>CPRFLKVKNWETDVVLTDTLHLKSTLETGCTEHICMGSIMLPSQHTRKPEDVRTKDQLFPLAKEFLDQYYSSIKRFGSKAHMDRLEEVNKEIESTSTYQLKDTELIYGAKHAWRNASRCVGRIQWSKLQVFDARDCTTAHGMFNYICNHVKYATNKGNLRSAITIFPQRTDGKHDFRVWNSQLIRYAGYKQPDGSTLGDPANVQFTEICIQQGWKAPRGRFDVLPLLLQANGNDPELFQIPPELVLEVPIRHPKFDWFK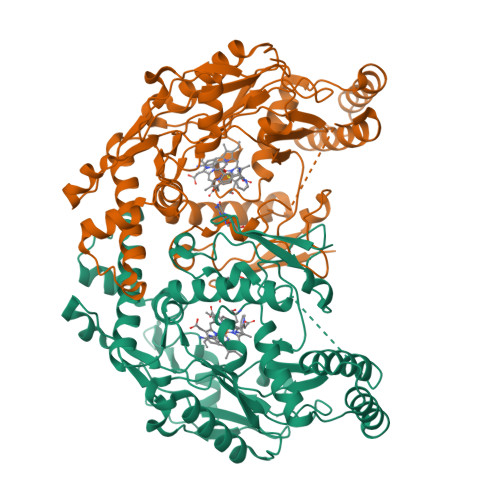DLGLKWYGLPAVSNMLLEIGGLEFSACPFSGWYMGTEIGVRDYCDNSRYNILEEVAKKMDLDMRKTSSLWKDQALVEINIAVLYSFQSDKVTIVDHHSATESFIKHMENEYRCRGGCPADWVWIVPPMSGSITPVFHQEMLNYRLTPSFEYQPDPWNTHVWKG[2x]> MKQYLELMQKVLDEGTQKNDRTGTGTLSIFGHQMRFNLQDGFPLVTTKRCHLRSIIHELLWFLQGDTNIAYLHENNVTIWDEWADENGDLGPVFGKQWRAWPTPDGRHIDQITTVLNQLKNDPDSRRIIVSAWNVGELDKMALAPCHAFFQFYVADGKLSCQLYQRSCDVFLGLPFNIASYALLVHMMAQQCDLEVGDFVWTGGDTHLYSNHMDQTHLQLSREPRPLPKLIIKRKPESIFDYRFEDFE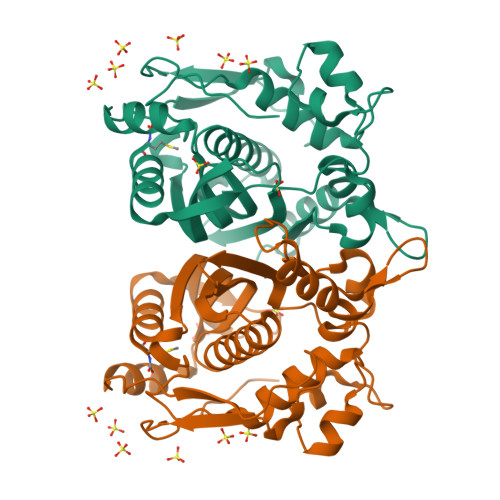IEGYDPHPGIKAPVAI>[2x]SLMADEIAKAQVARPGGDTIFGKIIRKEIPAKIIFEDDRCLAFHDISPQAPTHFLVIPKKHISQISVAEDDDESLLGHLMIVGKKCAADLGLNKGYRMVVNEGSDGGQSVYHVHLAVLGGRQMHWPPG

Diadenosine-5′,5-P1,P4-tetraphosphate (Ap4A) is a ubiquitous second messenger from bacteria to higher eukaryotes, which responds to environmental stresses and cell cycle phases. Ap4A then binds to the histidine triad nucleotide-binding protein 1 (HINT1), thereby disrupting the protein–protein interaction with microphthalmia-associated transcription factor (MITF), and the released MITF eventually promotes the transcription of mast cell activation genes. The HINT1 protein is a compact and symmetric dimer, with two adenosine pockets at opposite sides. Here we report that Ap4A specifically polymerizes HINT1 into (HINT1-Ap4A)n (HAn) filaments in solution and in the activated RBL cells.

We then made an H114A mutant to inactivate the hydrolysis activity of HINT1. The complex structures of HINT1H114A with Ap4A were then obtained through both co-crystallization (HINT1H114A-Ap4Acocrystallization, 0.95 Å) and soaking methods (HINT1H114A-Ap4Asoaking, 1.42 Å). The complete Ap4A molecule was observed in one adenosine pocket of a HINT dimer (denoted as HINT1 Dimer I) in both co-crystallization and soaking structures. The other adenosine pocket of the same HINT1 dimer is vacant of Ap4A, because it is blocked by the crystal packing. In both structures, one adenosine (A1) and the α-phosphate (Pα) of Ap4A bind inside the pocket, whereas the rest of the molecule adopts a unique Sticking-out conformation above the HINT1 surface. Interestingly, the Ap4A-complexed structure closely resembled the HINT1 apo structure with an overall RMSD about 0.238 Å. Only three positions including the residues S107, I32, and D16 surrounding the adenosine pocket had minor shifts of 1.3, 3.8, and 1.9 Å upon Ap4A binding. Of note, the sticking-out portion of Ap4A, containing the second adenosine (A2) and the delta phosphate (Pδ), fit into an adjacent HINT1 dimer in the crystal structure (denoted as HINT1 Dimer II). The two HINT1 dimers formed a large cleft with their adjoining adenosine pockets that accommodated Ap4A. Therefore, in the presence of Ap4A, two HINT1 dimers were integrated into a compact (HINT1)2-Ap4A-(HINT1)2 tetramer in the crystalline state.methyl 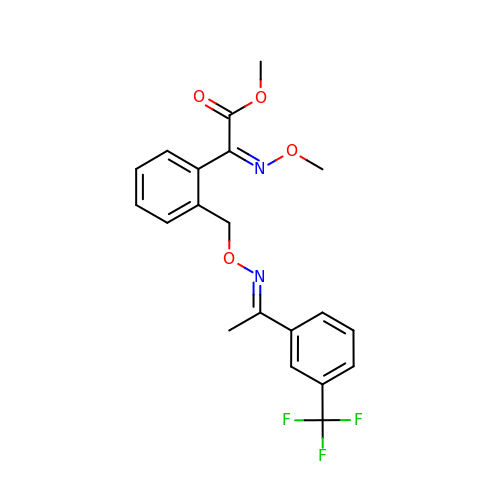(2E)-(methoxyimino)(2-{[({(1Z)-1-[3-(trifluoromethyl)phenyl]ethylidene}amino)oxy]methyl}phenyl)ethanoate | C20 H19 F3 N2 O4 | ONCZDRURRATYFI-KEEMFBDKSA-N In this work we have determined the structure of SpvD, a S. typhimurium SPI-2 T3SS effector protein that inhibits the NF-κB signaling pathway. In this work we determined the structure of SpvD and showed that it is a hydrolase with a papain-like fold and a catalytic triad composed of Cys-73, His-162, and Asp-182. Structurally, SpvD can be classified as belonging to the CA clan of cysteine proteases that contains papain and related proteases (MEROPS peptidase database). Although SpvD is highly conserved among different serovars of S. enterica, serovars Typhimurium and Enteritidis differ in containing an arginine or glycine, respectively, at residue 161 near the active site.

After unsuccessful crystallization of wild-type SpvD, we obtained crystals of SpvD in which its predicted surface cysteines were mutated (SpvDC37S/C122S/C160S/C170S, hereafter referred to as SpvD4CS), and these diffracted to 1.5 Å resolution. Subsequent structure determination revealed that SpvD adopts an α+β fold with a total of 7 α-helices, 6 β-strands, and a short stretch of 310 helix. Its central core is composed of a β-sheet formed by four antiparallel β-strands (β3–6) surrounded by five α-helices (α3–7). Additionally, there is a smaller β-sheet (β1–2) surrounded by α-helices 1–5. Close inspection of a shallow groove on the protein surface between helices α4/α5, strand β4, and the β5-α7 loop revealed a potential hydrolase active site including a catalytic triad of cysteine (Cys-73), histidine (His-162), and aspartic acid (Asp-182). The position of the superimposed five C-terminal amino acids of ubiquitin (RLRGG) is unobstructed in the SpvD4CS/G161/C73A variant (right), whereas in SpvD4CS/R161, binding would be impeded by the side chain of Arg-161, which restricts access to the active site (left). Therefore, the Arg-161 side chain could have an inhibitory steric or regulatory role in the activity of SpvD. Despite being less active in the DUB-GloTM assay, SpvDA154/R161 was the most active SpvD variant in the Ub-AML deconjugation assay. The fact that the SpvDR161 variant is present in all Salmonella serovars except Enteritidis, Bovismorbificans, and Abortus-equi is intriguing. It is possible that SpvDR161 has gained a different substrate specificity that is not related to NF-κB signaling.

> GPGMRVSGSASSQDIISRINSKNINNNDSNEVKRIKDALSIESKERILYPQNLSRDNLKQMARYVNNTYVHYSGNCVLLSACLHYNIHHRQDILSSKNTASPTVGLDSAIVDKIIFGHELNQSYSLNSIDEVEKEILNRYDIKRESSFIISAENYIAPIIGESRHDFNAVVISEYDKKPYVQFIDSWKTSNILPSLQEIKKHFSSSGEFYVRAYDEKHD>MESEGEAGAKPVTALGAQVCQICGDGVGKTVDGEPFVACDVCAFPVCRPCYEYERKDGNQSCPQCKTRYKRHKGSPAILGDMEEDGAAAADASDFNYDSENQNQNQNQKQKISERMLSWQLTYPRGEEVGAPNYDKDVSHNHIPLLTSGQEVSGELSAASPERLSMASPAVGGGKRVHNIPYSSDINQSPNIRAGDPGLGNVAWKERVDGWKMKQEKNVVPMSTGQAASERGAGDIDASTDVLVDDSLLNDEARQPLSRKVSIPSSRINPYRMVIMLRLVILCIFLHYRITNPVPNAYPLWLVSVICEIWFAISWILDQFPKWLPVNRETYLDRLALRYDREGEPSQLAAVDIFVSTVDPLKEPPLVTANTVLSILAVDYPVDKVSCYVSDDGAAMLTFEALAETSEFARKWVPFSKKYSIEPRAPEWYFSQKIDYLKDKVHPSFVKDRRAMKREYEEFKVRINGLVSKAQKVPEEGWVMQDGTPWPGNNTRDHPGMIQVFLGQSGGLDTEGNELPRLVYVSREKRPGFQHHKKAGAMNALVRVSAVLTNGPFLLNLDCDHYINNSKALREAMCFMMDPNLGKHVCYVQFPQRFDGIDRNDRYANRNTVFFDINLRGLDGIQGPVYVGTGCVFNRTALYGYEPPLKPKHKKPGLLSSLCGGTRKKSSKSSKKGSDKKKSSKHVDPTVPIFNLEDIEEGVEGTGFDDEKSLLMSQMSLEKRFGQSAVFVASTLMENGGVPQSATPETLLKEAIHVISCGYEDKTDWGSEIGWIYGSVTEDILTGFKMHARGWRSIYCMPKRPAFKGSAPINLSDRLNQVLRWALGSVEILFSRHCPIWYGYGGRLKWLERFAYVNTTIYPVTAIPLLIYCILPAVCLLTNKFIIPQISNLASIWFISLFLSIFATGILEMRWSGVGIDEWWRNEQFWVIGGVSAHLFAVFQGLLKVLAGIDTNFTVTSKASDEDGDFAELYMFKWTTLLIPPTTLLIINLVGVVAGISYAINSGYQSWGPLFGKLFFAFWVIIHLYPFLKGLMGRQNRTPTIVVVWSVLLASIFSLLWVRIDPFTTRVTGPDVEECGINC[3x]

Cellulose is synthesized by cellulose synthase (CesA), a membrane-integrated processive family-2 glycosyltransferase (GT; Lombard et al., 2014). The enzyme synthesizes cellulose from UDP-activated glucose (UDP-Glc) and translocates the polymer across the plasma membrane through a channel formed by its own membrane-spanning segment. While bacterial CesAs primarily function as monomeric enzymes, structural analyses of plant CesAs revealed their assembly into triangular-shaped trimeric complexes of three catalytically active subunits. Cryo-EM analyses of all three CesA isoforms reveal the formation of homotrimeric complexes, similar to the secondary cell wall CesAs.

The helix has been modeled for GmCesA1 and GmCesA6, while its density is detectable at a similar position but too discontinuous for modeling in the GmCesA3 map. TM helix 7 was excluded from the GmCesA3 model due to limiting map quality. The NTD has been resolved at lower resolution for PttCesA8, where it forms a helical stalk extending from the catalytic domains into the cytosol. We observe a similar stalk-like extension in some of the trimeric GmCesA3 particles. However, the NTD is only resolved for a small subset of GmCesA3 particles and not resolved at all for the other GmCesAs. This suggests that it can adopt multiple conformations, with the stalk being one of them. Our GmCesA3 structure contrasts with the recently reported dimeric organization of a fragment of A. thaliana’s (At) CesA3 catalytic domain, which self-associates via β-strand augmentation. Our cryo-EM analysis of GmCesA3 and the other isoforms only revealed monomeric and trimeric states, likely because the region involved in dimerization of the AtCesA3 fragment is inaccessible in the full-length GmCesA3 protein. GmCesA3 exhibits an activity optimum at pH 7 with a sharp decline at pH 8 and 9. Quantifying the release of UDP during biosynthesis reactions using a ‘UDP-Glo’ glycosyltransferase assay reveals Michaelis–Menten constants for GmCesA1 and GmCesA3 with respect to UDP-Glc of 0.44 mM and 0.18 mM, respectively.>MVLGYVSDMHTELASISQLVIAKIETIDNDILNKDIVNFIMCRSNLDNPFISFLDTVYTIIDQENYQTELINSLDDNEIIDCIVNKFMSFYKDNLENIVDAIITLKYIMNNPDFKTTYAEVLGSRIADIDIKQVIRENILQLSNDIRERYLGSKHHHHHH[8x]

VACV protein A49 prevents translocation of NF-κB to the nucleus by sequestering cellular β-TrCP, a protein required for the degradation of the inhibitor of κB. Unexpectedly, the structure showed that A49 possesses a Bcl-2-like fold despite not sharing sequence identity with known cellular or poxvirus Bcl-2 family proteins. Strikingly, despite a lack of sequence conservation with known family members, A49 adopts the Bcl-2 family protein fold comprising five α-helices wrapped around a central helix, α5 (45). The A49 structure shows that A49 lacks a surface groove compatible with binding BH3 peptides and is unable to bind the proapoptotic proteins Bax or Bak.

A truncated form of A49 lacking the N-terminal 12 amino acids (A49 Δ12) was thus expressed and purified. It crystallized readily in two distinct conditions, and diffraction data were recorded to 1.8–1.9 Å resolution (A49 Δ12 ammonium sulfate and A49 Δ12 sodium malonate). Residues 13–17 adopt three distinct conformations in the 10 A49 Δ12 molecules observed in the two crystal forms (inset) and are disordered in one of the two molecules of A49 Δ12 per asymmetric unit in crystals grown in the sodium malonate condition. In four of the eight molecules of A49 Δ12 grown in the ammonium sulfate condition and both molecules of A49 Δ12 grown in the sodium malonate condition, a single residue (Gly) of the C-terminal purification tag is observed; in the structure of full-length A49, the final two residues (161 and 162) and the purification tag were not ordered and could not be modeled. Visual inspection of the structures of A49 Δ12 and full-length A49 showed that, in all cases, two molecules of A49 self-associate via an interaction of helices α4 and α6 (the “4-6 face”). In the structure of full-length A49 this interaction is formed by crystallographic 2-fold symmetry, whereas in the structures of A49 Δ12 the interaction is formed by pseudo-2-fold non-crystallographic symmetry. In the structures of A49 Δ12 salt bridges Arg136–Asp92 and Lys103–Asp139 are formed, although these bonds are not symmetric and thus formed only once per pair of A49 molecules. In A49 Δ12 hydrogen bonds are formed between the side chains of Asn88 and Tyr102 and the carbonyl oxygens of Thr128 and Val95, respectively, and between the side chains of Arg136 and Asn96, although again these interactions often occur only once per pair of A49 molecules. Additionally, we observed that A49 crystallized much more readily upon removal of residues 1–12.> MGPSSGSRLGPPEAESPSQPPKRRKKRYLRHDKPPYTYLAMIALVIQAAPSRRLKLAQIIRQVQAVFPFFREDYEGWKDSIRHNLSSNRCFRKVPKDPAKPQAKGNFWAVDVSLIPAEALRLQNTALCRRWQNGGARGAFAKDLGPYVLHGRPYRPPSPPPPPSEGFSIKSLLGGSGEGAPWPGL

Forkhead box H1 (FoxH1) is an essential maternal pioneer factor during embryonic development that binds to specific GG/GT-containing DNA target sequences. The members of the FOX transcription factor family share the presence of the forkhead domain (FH), which interacts with DNA (InterPro entry IPR001766). Most FOX proteins recognize the canonical forkhead DNA motif TRTTTRY (R = A/G, Y = C/T). In contrast, FoxH1 recognizes the TGTG(G/T)ATT sequences in several cis-regulatory elements, such as in Gsc, Eomes, Nodal, Mixl, and FoxA2, to confer activin regulation in vivo.

To decipher how FoxH1 selects GK sites and how the extended domain contributes to DNA binding, we determined the crystal structures of FoxH1 proteins from three selected species, H. sapiens, D. rerio, and X. laevis, bound to a 16 bp native sequence belonging to the mouse Gsc promoter containing the GG site. The three GG complexes were refined at 0.98 Å (D. rerio, C2 space group), 1.47 Å (H. sapiens, P21 space group), and 2.8 Å resolution (X. laevis, P212121 space group). The root-mean-square deviations (RMSD) between the three vertebrate GG complexes range from 0.47 to 0.65 Å, indicating high structural conservation between the proteins. Although the human construct includes the engrailed homology 1 motif (EH1), this part is not defined in the complex, thereby suggesting that this region does not belong to the globular FH domain. Wing2 starts with two 310 helices (H4 and H5), followed by an isolated β-bridge formed by Lys185 and Asp202 in zebrafish and by Arg121 and Asp143 in humans. In the human and frog sequences, which are longer at the C-terminus, we detected a short coil fragment that turns back and runs antiparallel to H8. A comparison of the three GG complexes revealed the presence of a mammalian-specific insertion of five amino acids, 134-GlyGlyAlaArgGly-138, which is located within H7. This insertion cannot be accurately traced in the human structure due to intrinsic flexibility. At the 5′ site, these additional interactions occur through contacts from Lys104 (human sequence) or Lys168 (zebrafish) located in Wing1 with positions 2, 3, and 5 of DNA.>MHHHHHHMGSVLPELRRAQSLTCTGLYREALALWANAWQLQTQLGTPSGPDRPLLTLAGLAVCHQELEDPG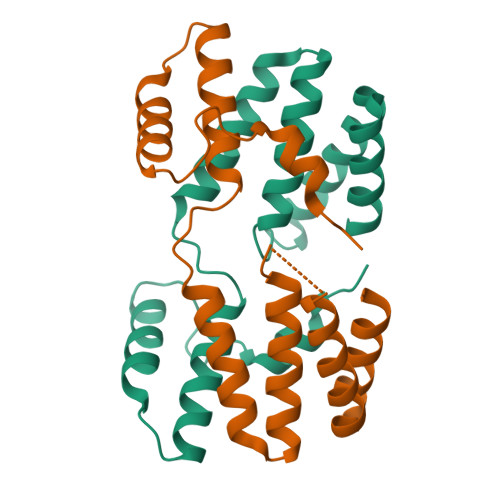EARACSEKALQLLGDKRPHPFLAPFLEAHVRLSWRLGLDKRQSEAQLQALQEAGLTSTPPPSLKELLIKEVLD[2x]> MGSSHHHHHHSSGLVPRGSSMEMIEKAPTDLEDRDKAPHLLLLAGIQGDEPGGFNATNLFLMHYSVLKGLVEVVPVLNKPSMLRNHRGLYGDMNRKFAALDKKDPEYPTIQEIKSLIAKPNIDAVLHLHDGGGYYRPVYVDAMLNPKRWGNCFIIDQDEVKGAKFPNLLAFANNTIESINAHLLHPIEEYHLKNTRTAQGDTEMQKALTFYAINQKKSAFANEASKELPLASRVFYHLQAIEGLLNQLNIPFKRDFELNPSSVHALINDKSLWAKISSLPKIPLFNLRPRLNHFPLPHNTKIPQIPIESNAYIVGLVKNKQEVFLKYGNKLMTRLSPFYIEFDPSLEEVKMQIDNKDQM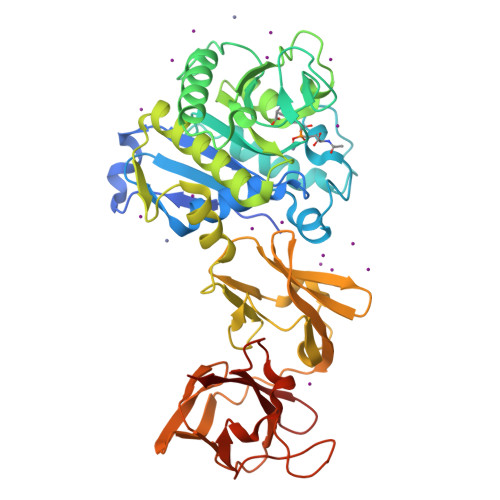VKIGSVVEVKESFYIHAMDNIRANVIGFSVSNENKPNEAGYTIRFKDFQKRFSLDKQERIYRIEFYKNNAFSGMILVKFV> SNAMPLPKSLKYGDTIGIYSPSSPVTYTSPKRFERAKSYLLQKGFHILEGSLTGRYDYYRSGSIQERAKELNALIRNPNVSCIMSTIGGMNSNSLLPYIDYDAFQNNPKIMIGYSDATALLLGIYAKTGIPTFYGPALVPSFG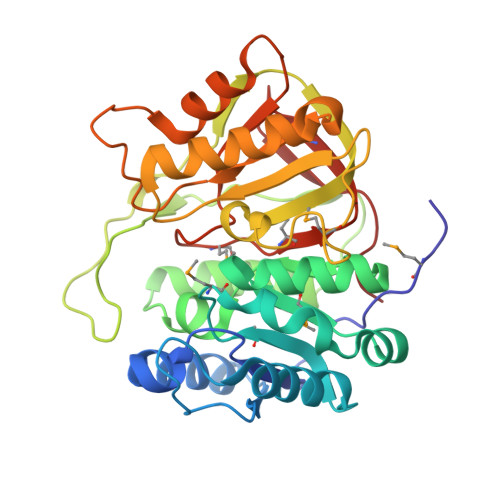EFEPFVDDTYKYFLETLLHDQALPYNIKQPLFWSDEFINWEEKTKEKELRPNNWISVTNGQATGRVIGGNLNTIQGIWGSPYMPCIQEGDILFIEDSSKDAATIERSFSFLKINGVFDKVSGIILGKHEQFDDCGTNRKPYEILLEVLQNQRIPLLADFDCCHTHPMITMPIGVQVKMDATNKTIHILEKWKI> MGSSHHHHHH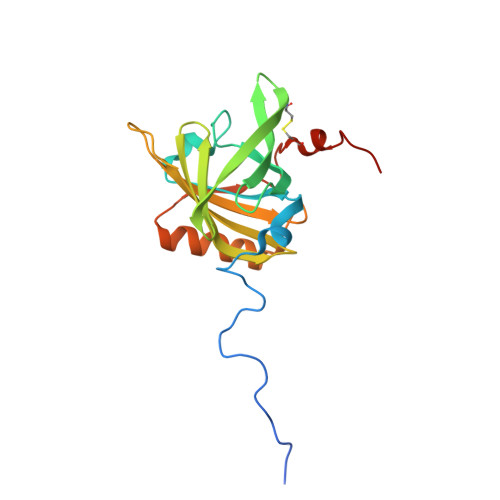SSGENLYFQGHMHEEENVVRSNIDISKISGEWYSILLASDVKEKIEENGSMRVFVEHIKALDNSSLSFVFHTKENGKCTEIFLVADKTKDGVYTVVYDGYNVFSIVETVYDEYILLHLLNFDKTRPFQLVEFYAREPDVSQKLKEKFVKYCQEHGIVNILDLTEVDRCLQARGSEVAQDSSV P. aeruginosa multidrug efflux Y (MexY) is an efflux pump that belongs to the resistance-nodulation-cell division (RND) superfamily. It is a major determinant for resistance to aminoglycosides in this opportunistic pathogen. MexY is also able to confer resistance to a range of other antimicrobial agents, such as fluoroquinolones, macrolides, tetracyclines, spectinomycin, chloramphenicol, and cefepime. This efflux pump is an inner membrane protein that works in conjunction with the MexX periplasmic membrane fusion protein and the OprM outer membrane channel to form the MexXY-OprM tripartite efflux system. It constitutes substrate-binding sites and utilizes the proton motive force (PMF) to export these antimicrobials out of the cell.

To further elucidate the molecular mechanisms of aminoglycoside-specific RND efflux pumps, here, we report the cryo-electron microscopy (cryo-EM) structure of the P. aeruginosa MexY aminoglycoside efflux pump to a resolution of 3.63 Å. The cryo-EM structure of MexY reveals that this multidrug efflux pump forms a homotrimer and adopts the overall fold of hydrophobe-amphiphile efflux (HAE)-RND membrane proteins. Similar to the assembly of many other HAE-RND pumps, the cryo-EM structure of MexY displays an asymmetric, homotrimeric architecture with the pseudo-threefold axis positioned perpendicular to the membrane surface. The conformational states of the three MexY protomers assembled to form this trimer can be assigned as “binding,” “resting,” and “extrusion” states (Fig. 2A through C), where the periplasmic cleft established between PC1 and PC2 of the "binding” conformer is open, but the periplasmic clefts in both the "extrusion" and "resting" conformers of this pump are closed. The MexY pump constitutes a large, spacious substrate-binding cavity deep inside the periplasmic cleft. This cavity, compartmentalized into the proximal and distal drug-binding sites, is surrounded with several anionic residues, such as E129, D133, and E175, and aromatic residues, including Y127, Y613, and Y659. Based on the structural information, these anionic and aromatic residues may be critically important for substrate recognition, where MexY may prefer to bind positively charged drugs. Within the “extrusion” protomer of MexY, the cryo-EM structure indicates a similar tunnel, where it vertically connects the opening situated at the ceiling of the central cavity up to the exit site located at the bottom of the funnel region of the MexY trimer. Like the extrusion tunnel of AcrD, this MexY extrusion tunnel is surrounded with charged residues such as D100, E129, K130, D133, R166, E169, K173, and E175. In addition to the extrusion tunnel, we noticed a formation of a horizontal tunnel at the “binding” protomer of MexY. This binding tunnel allows for the interior of the periplasmic domain of the “binding” protomer to be exposed to solvent via the entrance site of the periplasmic cleft created between subdomains PC1 and PC2.

>MARFFIDRPVFAWVISLLIVLAGVLAIRFLPVAQYPDIAPPVVNVSASYPGASAKVVEEAVTAIIEREMNGAPGLLYTKATSSTGQASLTLTFRQGVNADLAAVEVQNRLKIVESRLPESVRRDGIYVEKAADSIQLIVTLTSSSGRYDAMELGEIASSNVLQALRRVEGVGKVETWGAEYAMRIWPDPAKLTSMNLSASDLVNAVRRHNARLTVGDIGNLGVPDSAPISATVKVDDTLVTPEQFGEIPLRIRADGGAIRLRDVARVEFGQSEYGFVSRVNQMTATGLAVKMAPGSNAVATAKRIRATLDELSRYFPEGVSYNIPYDTSAFVEISIRKVVSTLLEAMLLVFAVMYLFMQNFRATLIPTLVVPVALLGTFTVMLGLGFSINVLTMFGMVLAIGILVDDAIIVVENVERLMAEEGLSPHDATVKAMRQISGAIVGITVVLVSVFVPMAFFSGAVGNIYRQFAVTLAVSIGFSAFLALSLTPALCATLLRPIDADHHEKRGFFGWFNRAFLRLTGRYRNAVAGILARPIRWMLVYALVIGVVALLFVRLPQAFLPEEDQGDFMIMVMQPEGTPMAETMANVGDVERYLAEHEPVAYAYAVGGFSLYGDGTSSAMIFATLKDWSERREASQHVGAIVERINQRFAGLPNRTVYAMNSPPLPDLGSTSGFDFRLQDRGGVGYEALVKARDQLLARAAEDPRLANVMFAGQGEAPQIRLDIDRRKAETLGVSMDEINTTLAVMFGSDYIGDFMHGSQVRKVVVQADGAKRLGIDDIGRLHVRNEQGEMVPLATFAKAAWTLGPPQLTRYNGYPSFNLEGQAAPGYSSGEAMQAMEQLMQGLPEGIAHEWSGQSFEERLSGAQAPALFALSVLIVFLALAALYESWSIPLAVILVVPLGVLGALLGVSLRGLPNDIYFKVGLITIIGLSAKNAILIIEVAKDHYQEGMSLLQATLEAARLRLRPIVMTSLAFGFGVVPLALSSGAGSGAQVAIGTGVLGGIVTATVLAVFLVPLFFLVVGRLFRLRKA[3x]> ANFLEHELSYIDVLLDKNADQATKDNLRSYFADKGLHSIKDIINKAK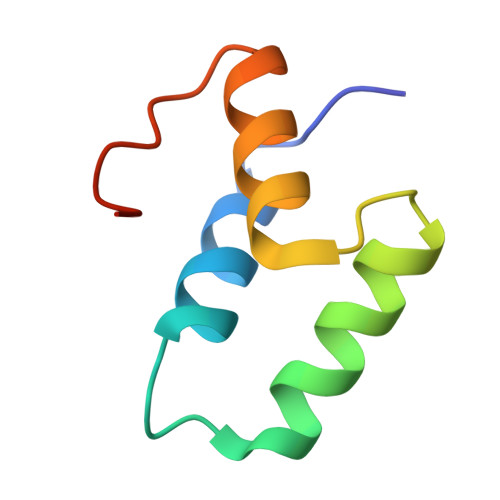QDGFDVSKYEHVK> LKQINHQGEEEELIALNLSEARLVIKEALVERRRAFKRSQKKHKKKHLKHENANDETTAVEDEDDDLD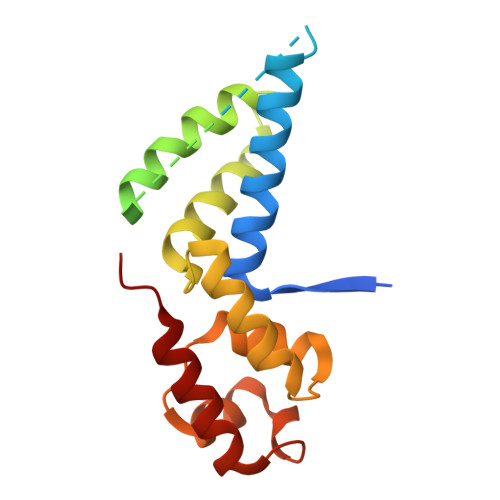EDDVNADDDDFMHSETREKELESIDVLLEQTTGGNNKDLKNTMQYLTNFSRFRDQETVGAVIQLLKSTGLHPFEVAQLGSLACDTADEAKTLIPSLNNKISDDELERILKELSNLETLY>[2x]MEHVAFGSEDIENTLAKMDDSQLD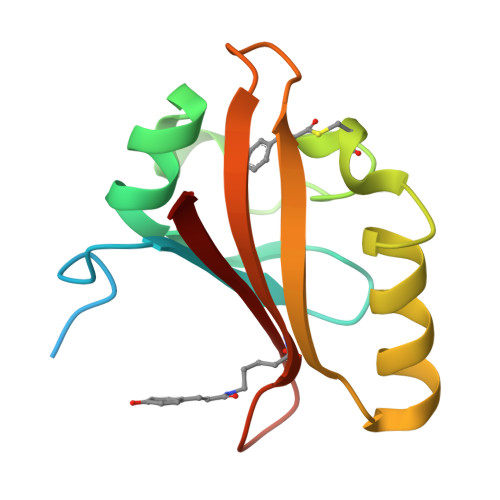NLAFGAIQLDGDGTILQYNAAEGDITGRNPKEVIGKNFFKDVAPCTDSPEFSGKFKEGVASGNLNTMFEYTFDYQMTPTKVKVHMKKALSGDSYWVFVKRV A major factor that limits the expansion of shrimp cultures is, however, infectious diseases from viruses, such as P. vannamei nodavirus (PvNV) and M. rosenbergii nodavirus (MrNV), which have inflicted heavy economic losses. The Nodaviridae genome comprises two single-stranded positive-sense RNA that encode the capsid protein for viral capsid assembly, the RNA polymerase for RNA replication, and the B2 protein for host RNA interference suppressor. While the shell domains (S-domains) of PvNV and MrNV contain conserved sequences of 62% identity, the protrusion domains (P-domains) and N-arms show low sequence identities of only 17% and 43%, respectively. In this work, we have determined the cryo-EM structures of T = 3 and T = 1 PvNV-LPs at atomic resolution, the crystal structures of the P-domains of PvNV and MrNV (PvNVPd and MrNVPd), and the crystal structure of the S-domain of PvNV (ΔN-ARM-PvNVSd) in the T = 1 subviral particle (SVP).

As for the MrNvPd, three crystal forms (P3221, C2221, and P4332) were determined. The overall conformations and dimer interfaces in three crystal structures of MrNVPd are similar with a RMSD < 0.3 Å. Second, the structure of MrNVPd (P4332) reveals an additional metal-binding site involved coordinating with both oxygen atoms from the side-chain carboxyl groups of two Glu300 residues. On the basis of the environment of the crystal condition, it is likely to be a divalent metal, such as cadmium (Cd2+). These two glutamic-acid residues from one MrNVPd dimer are conserved in PvNVPd (Glu302). The side chains of the two Glu300 residues on turn β3/β4 of the MrNVPd dimer alter the conformation upon coordinating the Cd2+ ions. The distances for the Cd2+-ligand oxygens from the two Glu300 residues are ~2.4 Å. Finally, the initial difference map shows one outstanding electron density peak near residues Cys309 and Thr343, which is interpreted as one Cd2+ ion. This Cd2+ ion is coordinated to the sulfur atoms from the side chain of Cys309 residue, one sulfate molecule from the crystallization buffer, and a backbone carbonyl oxygen atom from the main chain carboxyl groups from residues Thr343.

>[2x]PTPVEVSQLTYNADTIGNWVPPTELKQTYTQDITGLKPNSKFIIVPYMDRVSSEVLQKCTITCNEVDAVGSISYFDTSAIKCDGYISFQANSIGEATFTLVTDYQGAVDPKPYQYRIIRAIVGNN(2S)-2-[[(2S)-2-[(2-azanyl-4-oxidanylidene-1H-pteridin-7-yl)carbonylamino]-3-oxidanyl-propanoyl]amino]-3-(1H-indol-3-yl)propanoic 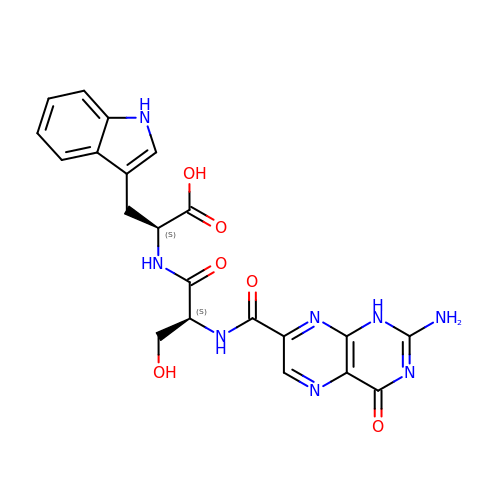acid | C21 H20 N8 O6 | PVENGVGTXKBGQJ-JSGCOSHPSA-N>MRPPLIERYRNLLPVSEKTPVISLLEGSTPLIPLKGPEEARKKGIRLYAKYEGLNPTGSFKDRGMTLAVSKAVEGGAQAVACASTGNTAASAAAYAARAGILAIVVLPAGYVALGKVAQSLVHGARIVQVEGNFDDALRLTQKLTEAFPVALVNSVNPHRLEGQKTLAFEVVDELGDAPHYHALPVGNAGNITAHWMGYKAYHALGKAKRLPRMLGFQAAGAAPLVLGRPVERPETLATAIRIGNPASWQGAVRA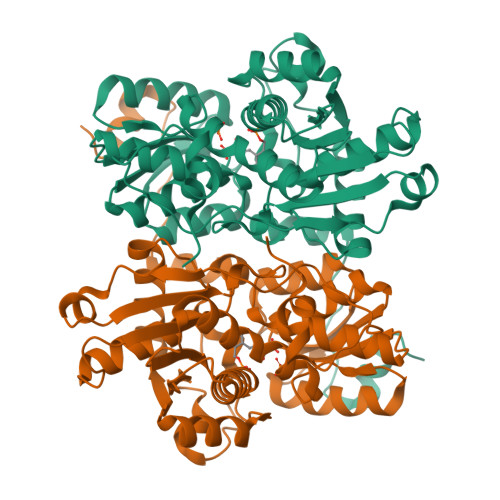KEESGGVIEAVTDEEILFAYRYLAREEGIFCEPASAAAMAGVFKLLREGRLEPESTVVLTLTGHGLKDPATAERVAELPPPVPARLEAVAAAAGLL[2x]>HMLLTTSRKPSQRTRSFSQRLSRIMGWRYINRGKMSLRDVLIEARGPVAVVSERHGNPARITFLDERGGERGYILFNPSFEMKKPELADKAVRVSSCPPGSEGLCNLMGLEVDESSSRDAWSIRT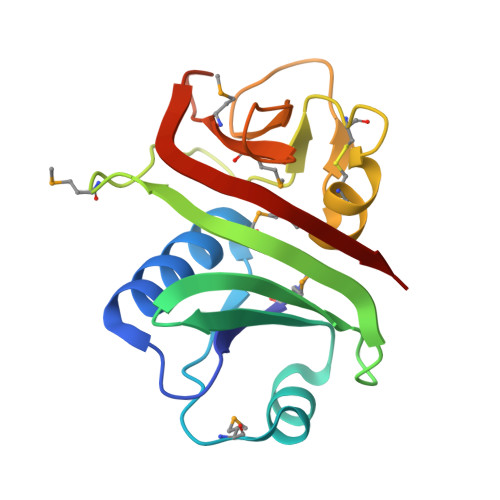DEEYAWVMELMDARGTPAGFKLLIRDFRVGE[2x]> MEGLAGYVYKAASEGKVLTLAALLLNRSESDIRYLLGYVSQQGGQRSTPLIIAARNGHAKVVRLLLEHYRVQTQQTGTVRFDGYVIDGATALWCAAGAGHFEVVKLLVSHGANVNHTTVTNSTPLRAACFDGRLDIVKYLVENNANISIANKYDNTCLMIAAYKGHTDVVRYLLEQRADPNAKAHCGATALHFAAEAGHIDIVKELIKWRAAIVVNGHGMTPLKVAAESCKADVVELLLSHADCDRRSRIEALELLGASFANDRENYDIIKTYHYLYLAMLERFQDGDNILEKEVLPPIHAYGNRTECRNPQELESIRQDRDALHMEGLIVRERILGADNIDVSHPIIYRGAVYADNMEFEQCIKLWLHALHLRQKGNRNTHKDLLRFAQVFSQMIHLNETVKAPDIECVLRCSVLEIEQSMNRVKNISDADVHNAMDNYECNLYTFLYLVCISTKTQCSEEDQCKINKQIYNLIHLDPRTREGFTLLHLAVNSNTPVDDFHTNDVCSFPNALVTKLLLDCGAEVNAVDNEGNSALHIIVQYNRPISDFLTLHSIIISLVEAGAHTDMTNKQNKTPLDKSTTGVSEILLKTQMKMSLKCL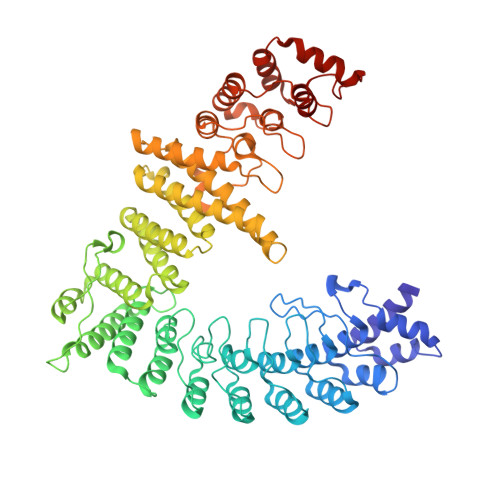AARAVRANDINYQDQIPRTLEEFVGFH>[6x]MAKHVVVIGGGVGGIATAYNLRNLMPDLKITLISDRPYFGFTPAFPHLAMGW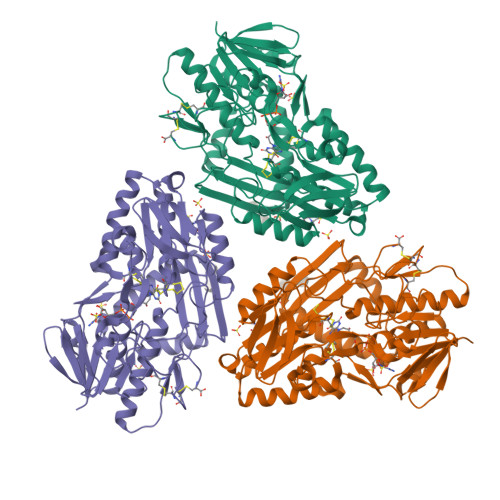RKFEDISVPLAPLLPKFNIEFINEKAESIDPDANTVTTQSGKKIEYDYLVIATGPKLVFGAEGQEENSTSICTAEHALETQKKLQELYANPGPVVIGAIPGVSCFGPAYEFALMLHYELKKRGIRYKVPMTFITSEPYLGHFGVGGIGASKRLVEDLFAERNIDWIANVAVKAIEPDKVIYEDLNGNTHEVPAKFTMFMPSFQGPEVVASAGDKVANPANKMVIVNRCFQNPTYKNIFGVGVVTAIPPIEKTPIPTGVPKTGMMIEQMAMAVAHNIVNDIRNNPDKYAPRLSAICIADFGEDAGFFFADPVIPPRERVITKMGKWAHYFKTAFEKYFLWKVRNGNIAPSFEEKVLEIFLKVHPIELCKDCEGAPGSRC3-{2-[(5-fluoro-2-hydroxyphenyl)amino]-1,3-thiazol-4-yl}benzonitrile 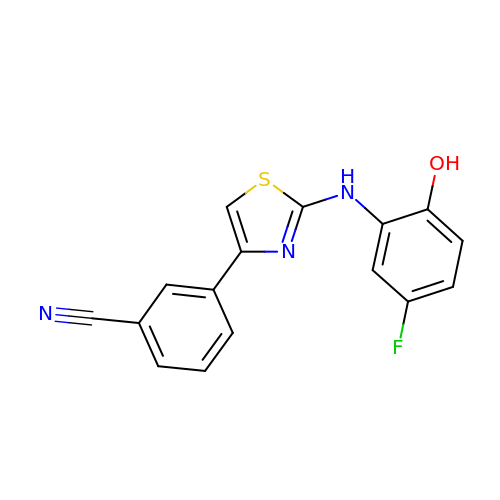| C16 H10 F N3 O S | WLSORBAAVBPTGJ-UHFFFAOYSA-N> KIPEHLIGKGAEADIKRDSYLD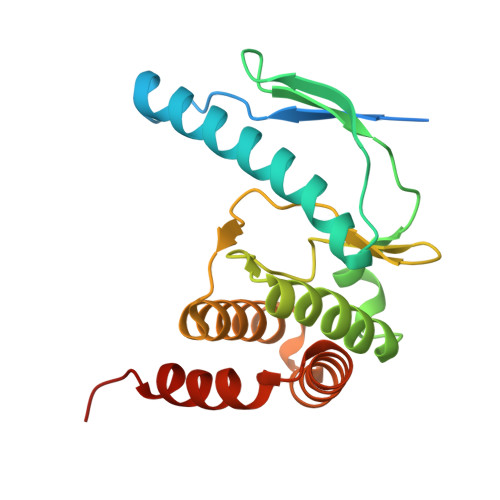FDVIIKERVKKGYRDERLDENIRKSRTAREARYLALVKDFGIPAPYIFDVDLDNKRIMMSYINGKLAKDVIEDNLDIAYKIGEIVGKLHKNDVIHNDLTTSNFIFDKDLYIIDFGLGKISNLDRDKAVDLIVFKKAVLSTHHEKFDEIWERFLEGYKSVYDRWEIILELMKDVERRARYVE Drosophila PGRP-LB belongs to the amidase PGRPs and downregulates the immune deficiency (IMD) pathway by cleaving meso-2,6-diaminopimelic (meso-DAP or DAP)-type PGN. The structure of the PGRP domain comprises three α-helices and one central β-sheet composed of six β-strands, similar to the bacteriophage T7 lysozyme, a zinc-dependent amidase. The main difference between amidase and non-catalytic PGRPs is the presence of Zn2+ in only amidase PGRPs, which is coordinated by two histidines and one cysteine. We generated mutants to characterize the amidase reaction mechanism and solved the X-ray structures of wild-type Drosophila PGRP-LBPA/PC and its mutants in apo form or complexed to TCT.

Structural analysis of Drosophila PGRP-LB and T7 Lysozyme, along with a multiple sequence alignment of PGRPs from different organisms, reveal the highly conserved residues of Drosophila PGRP-LBPA/PC histidine 42 (H42), histidine 152 (H152), tyrosine 78 (Y78) and cysteine 160 (C160) in coordination with Zn2+ in the catalytic site. In both structures, the Zn2+ is coordinated by H42, H152 and C160. In solution, one should expect that a water molecule would interact with both the residue Y78 and Zn2+ like in the T7 Lysozyme structure (Y46 and Zn2+). Additionally, the presence or absence of Zn2+ was assessed by X-ray emission fluorescence on PGRP-LBPA/PC wild type, Y78F and C160S crystals. We showed that Zn2+ is totally absent in PGRP-LBPA/PC_C160S mutant as already observed in the structure resolution, while it is still present in PGRP-LBPA/PC_Y78A mutant and PGRP-LBPA/PC wild type. Noticeably, no Zn2+ was added to the buffer during purification and crystallization steps, meaning that the Zn2+ present in the active site of PGRP-LBPA/PC_Y78A and PGRP-LBPA/PC proteins comes from the expression cell system. Of note, in the wild-type PGRP-LBPA/PC and PGRP-LBPD even without any Zn2+ in the media, the activity remains the same confirming the strong chelation of Zn2+ by the protein.

> GPMQQANLGDGVATARLLSRSDWGARLPKSVEHFQGPAPYVIIHHSYMPAVCYSTPDCMKSMRDMQDFHQLERGWNDIGYSFGIGGDGMIYTGRGFNVIGAHAPKYNDKSVGIVLIGDWRTELPPKQMLDAAKNLIAFGVFKGYIDPAYKLLGHRQVRDTECPGGRLFAEISSWPHFTHINDTEGVSSTTAPVVPHVHPQAAAPQKPHQSPPAAPKV> FMVSLPRMVYPQPKVLTPCRKDVLVVTPWLAPIVWEGTFNIDILNEQFRLQNTTIGLTVFAIKKYVAFLKLFLETAEKHFMVGHRVHYYVFTDQPAAVPRVTLGTGRQLSVLEVGAYKRWQDVSMRRMEMISDFCERRFLSEVDYLVCVDVDMEFRDHVGVEILTPLFGTLHP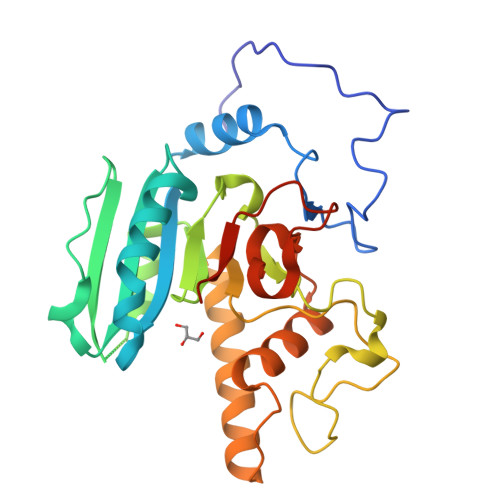SFYGSSREAFTYERRPQSQAYIPKDEGDFYYMGAFFGGSVQEVQRLTRACHQAMMVDQANGIEAVWHCESHLNKYLLRHKPTKVLSPEYLWDQQLLGWPAVLRKLRFTAVPKNHQAVRNPE> GPERIKGFNISGCSTKKLLWTYSTRSEEEFVLFCDLPEPQKSHFCHRNRLSPKQVPEHLPFMGSNDLSDVQWYQQPSNGDPLEDI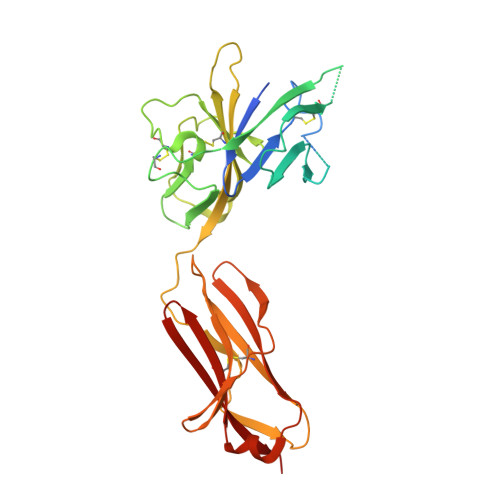RKSYPHIIQDKCTLHFLTPGVNNSGSYICRPKMIKSPYDVACCVKMILEVKPQTNASCEYSASHKQDLLLGSTGSISCPSLSCQSDAQSPAVTWYKNGKLLSVERSNRIVVDEVYDYHQGTYVCDYTQSDTVSSWTVRAVVQVRTIVGDTKLKPDILDPVEDTLEVELGKPLTISCKARFGFERVFNPVIKWYIKDSDLEWEVSVPEAKSIKSTLKDEIIERNIILEKVTQRDLRRKFVCFVQNSIGNTTQSVQLKEKR>SMDLKGLLHEENELPSIEKRKIDENAVEHDKVERKRTKSVAVPKIEMNFLNKPIVPDTTKVISNFLTHYLITEPVEHVEIEAKLGTLIDLETQNRFEFPVMNETILNPEFNLRTRFESDMTASEHKYLNEFLNQAFRDSQKPGRLPFAYKHTKQVDLFYETEDNSRDKIRVSKNQSDNQVLACVKKRRVADLFLYCPNDAFDIRISISDELPVSMPSGNQQPSLTRLKDRVGYVHQEIKIDLTKTTQNDPVYDTTERHELEVEFGNIADLRDRAQKAKDGMEAPLFRRVQLFMDN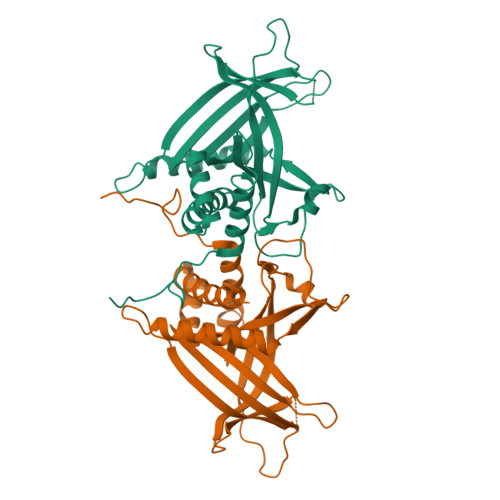VRILRREHS[4x]N-{[5-(4-fluorophenyl)-1H-pyrazol-4-yl]methyl}-N-methylethane-1,2-diamine | C13 H17 F N4 | 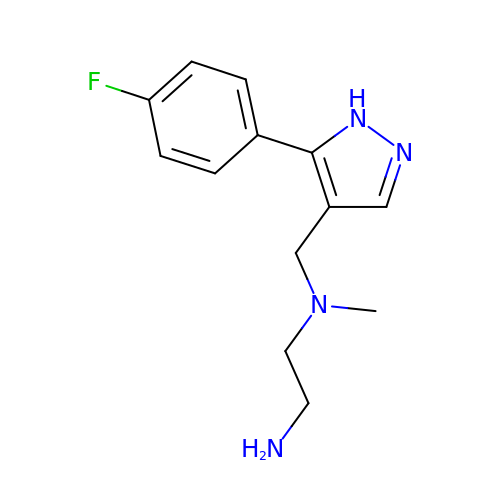WJJPSVIYQWOSFK-UHFFFAOYSA-N> MGSSHHHHHHSSGENLYFQGHMEAIQTHPANAAQAKAFTAPGSLSFPGGASEIANSTAPTNGASNGGQQQGVQATSGAGVTPATPAATPGAGPAGPSGITPTLQNIVATVNLDCRLDLKTIALHARNAEYNPKRFAAVIMRIREPKTTALIFASGKMVVTGAKSEDDSKLASRKYARIIQKLGFNAKFTDFKIQNIVGSCDIKFPIRLEGLASKHHNFSSYEPELFPGLIYRMIKPKIVLLIFVSGKIVLTGAKVREEIYQAFEMIYPVLQDFRKV;> MATRLDRLVTILETGSTRLIRDTAVNQLADWQKQHPEELFNLLSRVVPYLRHKDWETRTTAAKAIGKIIENAPLYDPNAGQDEAAPEPTNGSFEVKKEEEKDVLEQDNFFRLESLDVATIVKYGRPLLRGGPVDYNLAALDPQKRLAHLKKTLNGRLGLLGRVFEDEEMPVEQIASPITPNDAAGANGVGRQDGASNDNQSQAIDESKMSARQLNVLKRKRKREAQKAAQGKSGFGDLSLRRSTTAGSDAFGEDTPMPDADSKKNKLAEYFSLDRPENTEEDTKIVSEFKGPVLPIKSEIEADDSLEGAEWPFERLCEFLKVDLFDPQWETRHGAAMGLREVIRVHGAGAGRRRGKTRKENNDLNRQWLDDLAYRLLCVLMLDKFTDYSSDTSVAPIRETVGQTLGAVLRHISVESVHAIYRLLYCMVTQEDLPSEQNMWAVCHGGMVGLRYVVAVRKDLLLQDGDMIDGVVRCVMQGLGDIDDDVRSVSAATLIPMAKEFVMMRRSALDSLINIVWESLSNLGDDLSASTGKIMDLLATLCSFPEVLEAMKVSASQDEERSFTLLVPRLYPFLRHTITSVRLAVLKALMTFANLGGETSQGWLNGRILRLIFQNIIVERDQDTLNMSLELWTTLVRRLAARDPAILADEFEAHAEPMMQLALHPIGVPRHPIPMNPALFQKPSGGTYSLPGASQTNSRRSSPPEGERATKRRRKSTKAEDVAPSTHTHDVDGHMIQGEVDLVGVDVLIRSRISAAKAMGLIMSFIPTPRLASYDTAVLQALSSPYASTQLAAAMVIDEYAKNCSTPEVASRFIEPLQKIIDLERPSHYRDLVTYVQRVRSASQQLINLFRDHGKVSQGKLPTLAVVVQGEPEAGPGAFSIANAEKVVNEDFERLKRLMAPGQRLIALPQLNEAREQTVEVIEEAKAAKEARDARIKAAAACALVAMKVLPKKPSPLIKAIMDSIKTEENQELQSRSAATIARLVQLFTESGRRGPAEKVVANLVKFSCVEVAETPEFPIHAHKTNVILSMQKEEDRVDHPDAVKYAREAKAARITRRGAKEALEILSKNFGAELLERVPTLRTFMEEPLVRAFSGDLPPEARDPENAFGQEIVDAMSVIRTMTPTLHPALHPFVMQQVPLVIKALRSDLSVFRYMAAKCMATICSVITVDGMTALVEKVLPSINNPLDLSFRQGAIEVIYHLIAVMGDAILPYVIFLIVPVLGRMSDSDNQIRLIATTSFATLVKLVPLEAGIPDPPGLSEELLKGRDRERTFIAQLLDPKKIEPFKIPVAIKAELRSYQQEGVNWLAFLNKYHLHGILCDDMGLGKTLQTICIVASDHHQRAEEFARTGAPEVRKLPSLIICPPTLSGHWQQEIKTYAPFLTVTAYVGSPAERRAMKDSLDKTDIVITSYDVCRNDIDVIEKYNWNYCVLDEGHLIKNPKAKITLAVKRLTSNHRLILTGTPIQNNVLELWSLFDFLMPGFLGAEKVFLDRFAKPIANSRYSKASSKEQEAGALAIEALHKQVLPFLLRRLKEEVLNDLPPKILQNYYCDLSDLQRKLFEDFTKREGKKITETAGRDDKEAKQHIFQALQYMRKLCNSPALVMKPGHKAYEDTQKYLAKHGTTLEDPIHAPKLGALRDLLVDCGIGVEGQESSDPLYTPIKPHRALIFCQMKEMLDMVQNTVLKQMLPSVSYLRLDGSVEANKRQDIVNKFNSDPSYDVLLLTTSVGGLGLNLTGADTVIFVEHDWNPQKDLQAMDRAHRIGQKKVVNVYRIITRGTLEEKILSLQRFKIDVASTVVNQQNAGLATMDTDQILDLFNLGESGPSLITDNKESIEGREED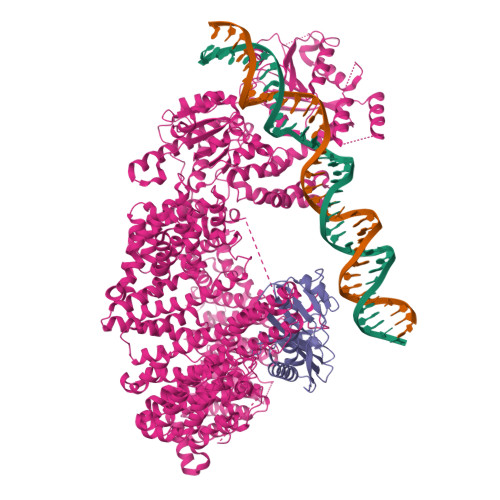MVDIETGDVRRPGKKAAWLEGLGELWDNAQYEESFDLDGFLKTMQAAAWSHPQFEK>DDHS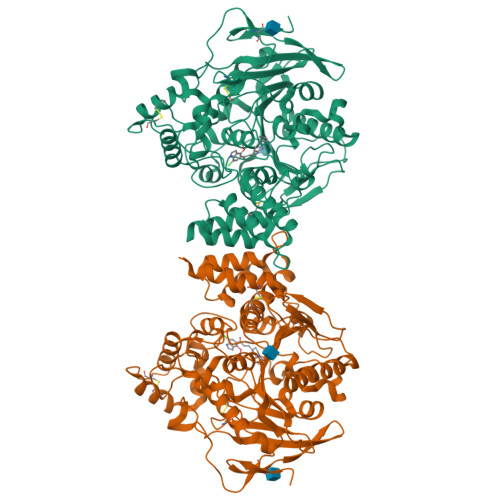ELLVNTKSGKVMGTRVPVLSSHISAFLGIPFAEPPVGNMRFRRPEPKKPWSGVWNASTYPNNCQQYVDEQFPGFSGSEMWNPNREMSEDCLYLNIWVPSPRPKSTTVMVWIYGGGFYSGSSTLDVYNGKYLAYTEEVVLVSLSYRVGAFGFLALHGSQEAPGNVGLLDQRMALQWVHDNIQFFGGDPKTVTIFGESAGGASVGMHILSPGSRDLFRRAILQSGSPNCPWASVSVAEGRRRAVELGRNLNCNLNSDEELIHCLREKKPQELIDVEWNVLPFDSIFRFSFVPVIDGEFFPTSLESMLNSGNFKKTQILLGVNKDEGSFFLLYGAPGFSKDSESKISREDFMSGVKLSVPHANDLGLDAVTLQYTDWMDDNNGIKNRDGLDDIVGDHNVICPLMHFVNKYTKFGNGTYLYFFNHRASNLVWPEWMGVIHGYEIEFVFGLPLVKELNYTAEEEALSRRIMHYWATFAKTGNPNEPHSQESKWPLFTTKEQKFIDLNTEPMKVHQRLRVQMCVFWNQFLPKLLNATAC[2x]While sequence analysis suggests that LsrF will function as a class I aldolase and genetic data suggests LsrF is involved in P-AI-2 processing, the details of the role LsrF plays in processing P-AI-2 are not known. To begin addressing this question, we have determined the crystal structure of LsrF, alone and in complex with the P-AI-2 analogues ribose-5-phosphate and ribulose-5-phosphate. LsrF crystallizes as a decamer with each monomer having an (αβ)8-barrel fold, a ubiquitous fold commonly seen in proteins catalyzing aldolase reactions. The LsrF oligmer has a disk-like structure, with two rings of five monomers stacked on top of each other giving rise to a decamer with D5 symmetry.

In a departure from the typical (αβ)8-barrel fold, the first β-strand of the LsrF barrel does not start until residue 51. Instead, the first 25 residues of the chain extend away from the barrel and pack against other subunits in a form of domain swapping previously unseen in aldolases. Monomers stacked on top of each other have extensive interactions that are significantly enhanced by a ‘swapping’ of N-terminal residues. In this swap, residues 10–24 extend away from the (αβ)8-barrel formed by their chain and pack into the interface between two adjacent monomers in the other pentamer, burying 460 Å2, or 21% of the accessible surface area of this swapped coil. When all of the interfaces are considered, approximately 40% of the total surface area is buried in oligomer formation, suggesting that the decamer is likely the predominant form of LsrF in vivo. Consistent with this conclusion, only decamers were observed in gel filtration experiments (data not shown). A single water was built in the binding site of unliganded LsrF; this water is displaced upon ligand binding. Structural alignments of LsrF with a variety of type I aldolases, including FBP aldolase from rabbit and T. tenax, ADH synthase from M. jannaschii, and transaldolase B, DERA, and 2-keto-3-deoxy-6-phosphogluconate (KDPG) from E. coli show structural conservation of the catalytic lysine with LsrF K203. The aspartic acid is then thought to donate the proton back during the reforming of the imine. This asparate is structurally conserved in LsrF (Asp57) and is well positioned to participate in catalysis as a general acid/base. Rather, there is an aspartate (251) located only 2.9 Å from the K203, though on the other side of the lysine from the catalytic glutamate in rabbit FBP aldolase.

>GSMADLDDIKDGKDFRTDQPQKNIPFTLKGCGALDWGMQSRLSRIFNPKTGKTVMLAFDHGYFQGPTTGLERIDINIAPLFEHADVLMCTRGILRSVVPPATNRPVVLRASGANSILAELSNEAVALSMDDAVRLNSCAVAAQVYIGSEYEHQSIKNIIQLVDAGMKVGMPTMAVTGVGKDMVRDQRYFSLATRIAAEMGAQIIKTYYVEKGFERIVAGCPVPIVIAGGKKLPEREALEMCWQAIDQGASGVDMGRNIFQSDHPVAMMKAVQAVVHHNETADRAYELYLSEKQ[20x]> GAGCACCTGTA;> ACACCGT;> CTGACTGTGGTGC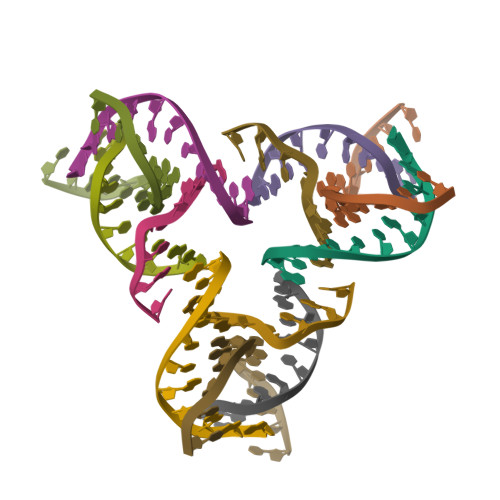T;> CGGACAGTCA>MSIKTTRDRVPTYQYNMNFEKLGKCIIINNKNFDKVTGMGVRNGTDKDAEALFKCFRSLGFDVIVYNDCSCAKMQDLLKKASEEDHTNAACFACILLSHGEENVIYGKDGVTPIKDLTAHFRGDRCKTLLEKPKLFFIQACRGTELDDGIQAASGPINDLVPRGSTDANPRYKIPVEADFLF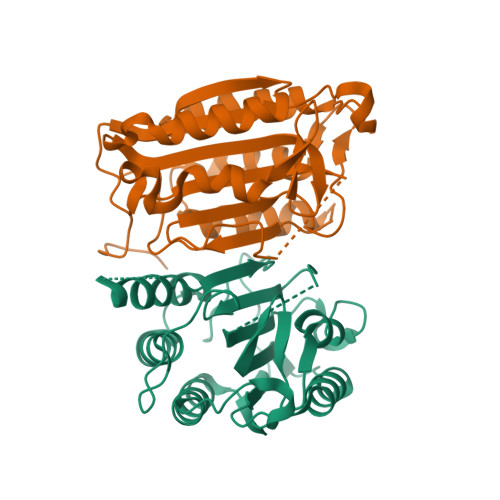AYSTVPGYYSWRSPGRGSWFVQALCSILEEHGKDLEIMQILTRVNDRVARHFESQSDDPHFHEKKQIPCVVSMLTKELYFSQLEHHHHHH[2x]>MKLYMSVDMEGISGLPDDTFVDSGKRNYERGRLIMTEEANYCIAEAFNSGCTEVLVNDSHSKMNNLMVEKLHPEADLISGDVKPFSMVEGLDDTFRGALFLGYHARASTPGVMSHSMIFGVRHFYINDRPVGELGLNAYVAGYYDVPVLMVAGDDRAAKEAEELIPNVTTAAVKQTISRSAVKCLSPAKRGRLLTEKTAFALQN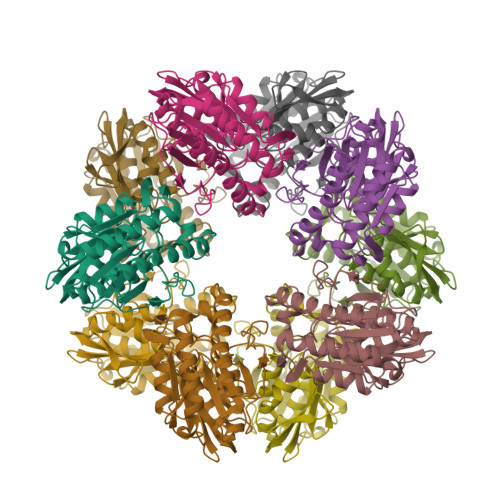KDKVKPLTPPDRPVLSIEFANYGQAEWANLMPGTEIKTGTTTVQFQAKDMLEAYQAMLVMTELAMRTSFC[5x]>[2x]SNAMLRRLFKKKYVCVRQYDLTDCGAACLSSIAQYYGLKMSLAKIREMTGTDTQGTNAYGLIHAAKQLGFSAKGVKASKEDLLKDFRLPAIANVIVDNRLAHFVVIYSIKNRIITVADPGKGIVRYSMDDFCSIWTGGLVLLEPGEAFQKGDYTQNMMVKFAGFLKPLKKTVLCIFLASLLYTALGIAGSFYIKFLFDDLIKFEKLNDLHIISAGFAVIFLLQIFLNYYRSILVTKLGMSIDKSIMMEYYSHVLKLPMNFFNSRKVGEIISRFMDASKIRQAISGATLTIMIDTIMAVIGGILLYIQNSSLFFISFIIILLYGIIVTVFNKPIQNANRQIMEDNAKLTSALVESVKGIETIKSFGAEEQTEKSTRDKIETVMKSSFKEGMLYINLSSLTGIVAGLGGIVILWAGAYNVIKGNMSGGQLLAFNALLAYFLTPVKNLIDLQPLIQTAVVASNRLGEILELATEKELREDSDDFVISLKGDIEFRNVDFRYGLRKPVLKNINLTIPKGKTVAIVGESGSGKTTLAKLLMNFYSPEKGDILINGHSIKNISLELIRKKIAFVSQDVFIFSGTVKENLCLGNENVDMDEIIKAAKMANAHDFIEKLPLKYDTFLNESGANLSEGQKQRLAIARALLKKPDILILDEATSNLDSITENHIKDAIYGLEDDVTVIIIAHRLSTIVNCDKIYLLKDGEIVESGSHTELIALKGCYFKMWKQTENTLAS;>[2x]SNAMSEAKKLNIGRELTDEELMEMTGGSTFSIQCQKDYTYKPSLPVVKYGVVIDEPEVVIKYGVGPIVGIKYGVEPIGPIQPMYGIKPVETLK

Peptidase-containing ABC transporters (PCATs) in gram-positive bacteria function both as maturation proteases and exporters for biofilm formation, quorum sensing, or antimicrobial polypeptides. Substrates of PCATs are synthesized as precursors with an N-terminal leader peptide. Proteolytic cleavage of the leader peptide at the conserved double-glycine motif is necessary for secretion of the cargo peptide. In this work, we determined the structures of wild-type PCAT1 (wtPCAT1) in the presence of substrate and ATP with or without Mg2+.

To analyze the conformational states of PCAT1 under ATP turnover conditions, cryo-EM samples were prepared using wtPCAT1 mixed with twofold molar excess of the substrate CtA, 10 mM ATP-Mg2+, and the creatine phosphate ATP-regenerating system. Among the 671,000 particles analyzed by three-dimensional (3D) classification, ∼83% exhibit IF conformations with different degrees of NBD separation, 14% are in an NBD-dimerized configuration, and the remaining 3% do not show any protein features. Subsequent refinement resulted in a low-resolution (6.6-Å) NBD-dimerized structure and three molecular structures of NBD-separated IF conformations, referred to as IF wide (IFW, 4.1 Å), intermediate (IFI, 3.7 Å), and narrow (IFN, 3.7 Å), respectively. The three IF structures share a similar overall conformation, in which the two PEP domains dock symmetrically onto the intracellular openings of the TM cavity. The leader peptide (residues 8 to 24) of the substrate forms an L-shaped structure wrapping around the PEP domain. The double-glycine cleavage site (G23/G24) is positioned on a narrow cleft on PEP in close proximity to the catalytic triad residues C21, H99, and D115. Consistently, the density inside the TM cavity is separated from both leader peptides, indicating that the cargo peptide inside the TM cavity has been freed from its leader peptide. Densities consistent with ATP and Mg2+ were observed in all three reconstructions. Different from the NBD-dimerized structure, in the NBD-separated conformations, ATP binds to the Walker A/B motifs of one NBD, distant from the ABC signature motif of the opposite NBD. The majority of PCAT1 adopts an IF conformation in which the NBDs are separated, the substrate is enclosed inside the TM cavity, and the PEP domains remain associated with the transporter core.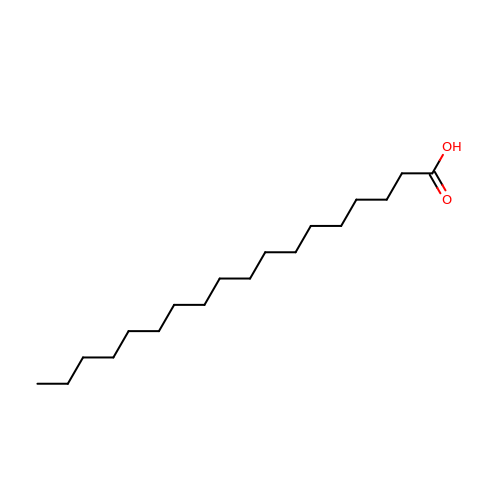STEARIC ACID | C18 H36 O2 | QIQXTHQIDYTFRH-UHFFFAOYSA-N2-[(9~{S})-7-(4-chlorophenyl)-4,5,13-trimethyl-3-thia-1,8,11,12-tetrazatricyclo[8.3.0.0^{2,6}]trideca-2(6),4,7,10,12-pentaen-9-yl]-~{N}-[2-[2-[2-[2-[2-[2-[2-[2-[2-[(9~{S})-7-(4-chlorophenyl)-4,5,13-trimethyl-3-thia-1,8,11,12-tetrazatricyclo[8.3.0.0^{2,6}]trideca-2(6),4,7,10,12-pentaen-9-yl]ethanoylamino]ethoxy]ethoxy]ethoxy]ethoxy]ethoxy]ethoxy]ethoxy]ethyl]ethanamide 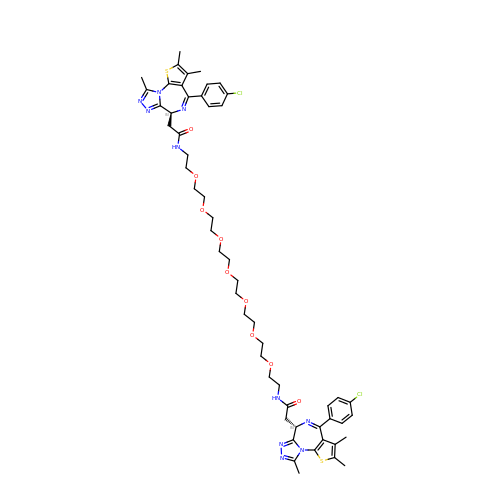| C54 H66 Cl2 N10 O9 S2 | JNSLBXJNVHYNNW-CXNSMIOJSA-N> GPGSNCGPPPTLSFAAPMDITLTETRFKTGTTLKYTCLPGYVRSHSTQTLTCNSDGEWVYNTFCIYKRCRHPGELRNGQVEIKTDLSFGSQIEFSCSEGFFLIGSTTSRCEVQDRGVGWSHPLPQ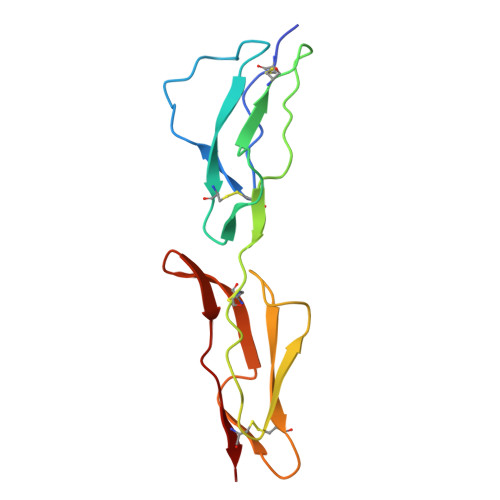CEI7-fluoro-4-(5-methyl-3H-imidazo[4,5-b]pyridin-6-yl)-2,4-dihydropyrazolo[4,3-b]indole 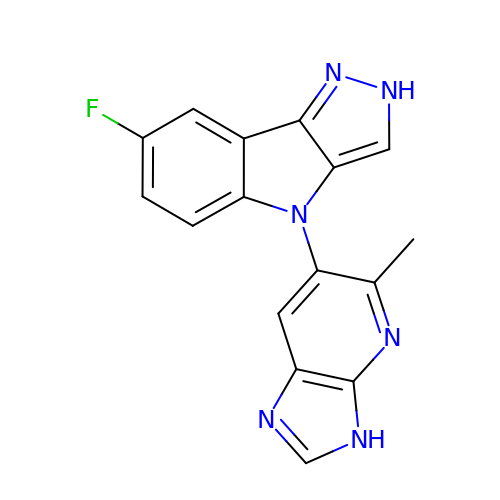| C16 H11 F N6 | BGVWCIRYUNODHW-UHFFFAOYSA-N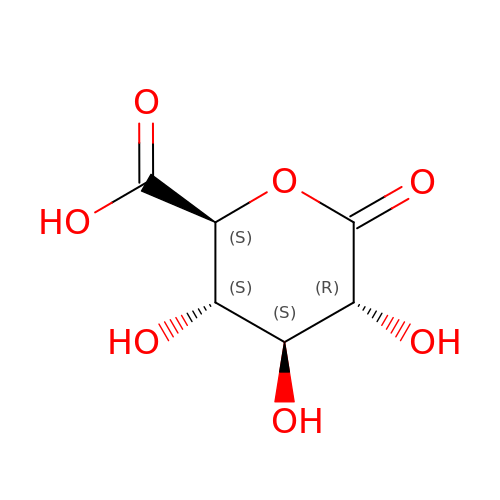(2S,3S,4S,5R)-3,4,5-trihydroxy-6-oxo-oxane-2-carboxylic acid | C6 H8 O7 | YLKFQNUGXOLRNI-QDQPNEQZSA-N(2R)-2,4-dihydroxy-3,3-dimethyl-N-[3-oxo-3-(pentylamino)propyl]butanamide | 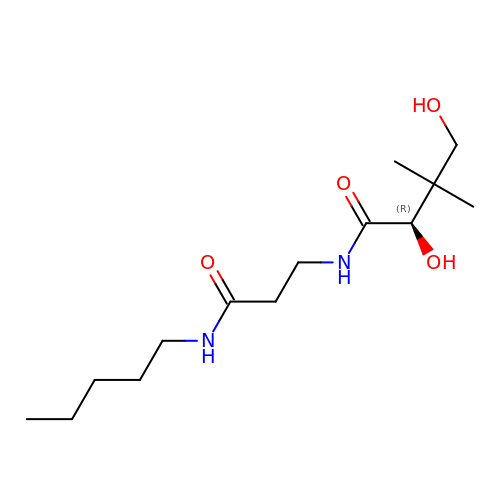C14 H28 N2 O4 | HWNKKPMQPCHGBA-LBPRGKRZSA-N>XALAA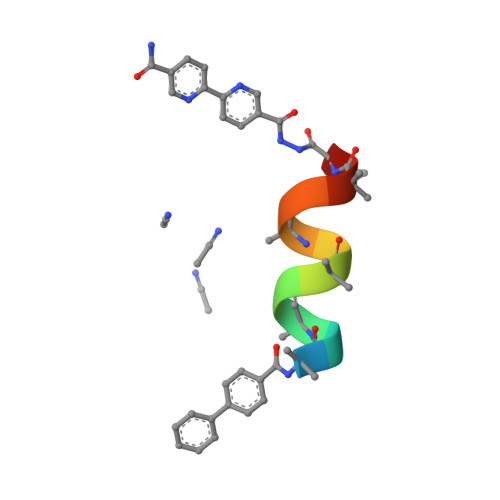ALAQALX[2x]>[2x]MAQAKHKQRKRLKSSCKRHPLYVDFSDVGWNDWIVAPPGYHAFYCHGECPFPLADHLNSTNHAIVQTLVNSVNSKIPKACCVPTELSAISMLYLDENEKVVLKNYQDMVVEGCGCR;>GSGAMAQNLDSMLHGTGMKSDSDQKKSENGVTLAPEDTLPFLKCYCSGHCPDDAINNTCITNGHCFAIIEEDDQGETTLTSGCLGLEGSDFQCRDTPIPHQRRSIECCRTNLCNQY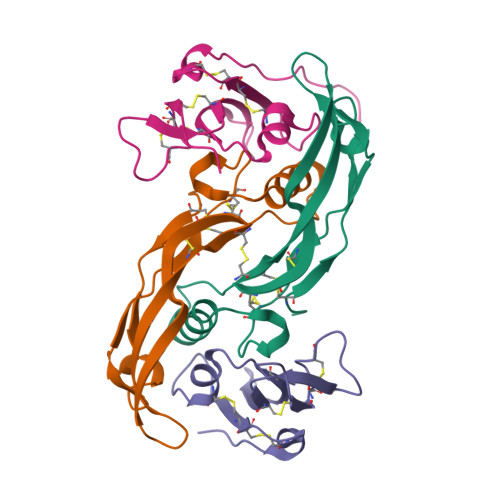LQPTLPPVVIGPFFDGSIR[2x]>[2x]MTSAEMTSPNNNSEHQAIAKMRTMIEGFDDISHGGLPIGRSTLVSGTSGTGKTLFSIQFLYNGIIEFDEPGVFVTFEETPQDIIKNARSFGWDLAKLVDEGKLFILDASPDPEGQEVVGGFDLSALIERINYAIQKYRARRVSIDSVTSVFQQYDASSVVRRELFRLVARLKQIGATTVMTTERIEEYGPIARYGVEEFVSDNVVILRNVLEGERRRRTLEILKLRGTSHMKGEYPFTITDHGINIFPLGAMRLTQRSSNVRVSSGVVRLDEMCGGGFFKDSIILATGATGTGKTLLVSRFVENACANKERAILFAYEESRAQLLRNAYSWGMDFEEMERQNLLKIVCAYPESAGLEDHLQIIKSEINDFKPARIAIDSLSALARGVSNNAFRQFVIGVTGYAK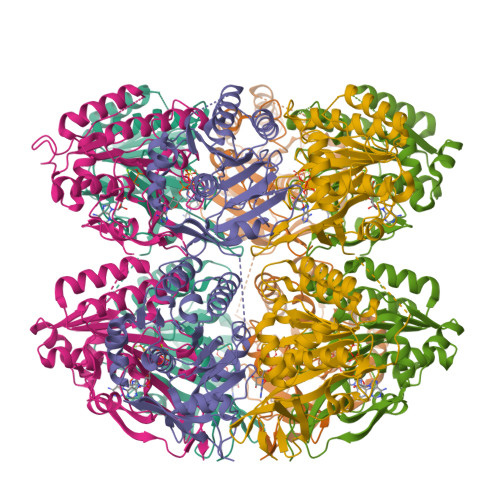QEEITGLFTNTSDQFMGAHSITDSHISVITDTIILLQYVEIRGEMSRAINVFKMRGSWHDKAIREFMISDKGPDIKDSFRNFERIISGSPTRITVDEKSELSRIVRGVQEKGPES V1 is a part of an ion pump V-ATPase, which transports cations across the membrane by ATP-hydrolysis-driven rotation. V1 comprises a rotor composed of the D and F subunits, and a stator, a hexameric ring, composed of three A subunits and three B subunits. However, the details of their sequences and structures are different, resulting in two different interfaces between the A and B subunits in the A3B3 hexameric ring: a catalytic interface, at which the A subunit has an ATP-hydrolysis catalytic site; and a non-catalytic interface, at which the B subunit has a pseudo-active site, which has evolutionally lost the ATP-hydrolysis or even binding ability. We used computational design to restore the lost ATP-binding ability of the pseudo-active site in the B subunit of a rotary molecular motor, V1-ATPase.

The designed B subunit (De), expressed together with the A subunit in Escherichia coli and purified by Ni2+-affinity chromatography followed by gel-filtration chromatography, was found to form a ring complex with the A subunit (A3(De)3 ring complex). Therefore, we determined the crystal structures of the A3(De)3 complex to prove the nucleotide-binding ability of De. First, the A3(De)3 complex was crystallized in the absence of nucleotide and the structure was solved at 2.8 Å resolution; this was named A3(De)3_empty. The De structure in A3(De)3_empty was almost identical to the computational model not only in terms of the overall structure but also in terms of the designed site together with the P-loop features. ADP molecules are shown as spheres. c,d, Superposition of the computational design model of the designed B subunit (white) and the solved crystal structure in the absence of nucleotides (pink) (chain D of A3(De)3_empty was used because this had the highest resolution data of the three designed B subunits): comparison for the entire backbone (the Cα r.m.s.d. calculated by MICAN33 is 1.48 Å) (c); comparison for the designed binding site (d). The backbone geometry of the designed P-loop was almost identical to that of the design model. e, The interface between chains C and D in A3(De)3_(ADP·Pi)1cat(ADP)2cat,2non-cat.

>SSGMQIGKIIKVSGPLVMAENMSEASIQDMCLVGDLGVIGEIIEMRQDVASIQVYEETSGIGPGEPVRSTGEALSVELGPGIISQMFDGIQRPLDTFMEVTQSNFLGRGVQLPALDHEKQWWFEATIEEGTEVSAGDIIGYVDETKIIQHKIMVPNGIKGTVQKIESGSFTIDDPICVIETEQGLKELTMMQKWPVRRGRPIKQKLNPDVPMITGQRVIDTFFPVTKGGAAAVPGPFGAGKTVVQHQIAKWSDVDLVVYVGCGERGNEMTDVVNEFPELIDPNTGESLMERTVLIANTSNMPVAAREASIYTGITIAEYFRDMGYDVAIMADSTSRWAEALREMSGRLEEMPGDEGYPAYLGSRLAEYYERSGRVIALGSDQREGSITAISAVSPSGGDISEPVTQNTLRVVKVFWGLDSSLAQKRHFPSINWIQSYSLYSTEVGRYMDQILQQDWSDMVTEGMRILQEEEQLNEIVRLVGIDSLSDNDRLTLEVAKSIREDYLQQNAFDDVDTFTSREKQFNMLKVILTFGKEARKALSLGAYFNEIMEGTVAVRERISRSKYIPEEELAKISSINEEIKETIQLIVSEGGMTDD[3x];>[3x]MIKEYRTIKEVVGPLMAVEKVSGVKYEELIEVRMQNGEIRRGQVLEVQEDKAMVQIFEGTSGINLKNSSVRFLGHPLQLGVSEDMIGRVFDGLGRPKDNGPEILPEKYLDINGEVINPIARDYPDEFIQTGISAIDHLNTLVRGQKLPVFGPPGAGKSALAAQIARQATVLDSSDDFAVVFAAIGITFEEAEFFMEDFRQTGAIDRSVMFMNLANDPAIERIATPRMALTAAEYLAYEKGMHVLVIMEDMTNYAEALREISAARREVPGRRGYPGYLYTNLATLFERAGRIRGLKGSVTQIPILTMPEDDKTHPIPDLTGYITEGQIILTRELYKSGISPPIDVLPSLSRLKDKGTGAGKTREDHAATMNQLFAAYAQGKQAKELAVVLGESALSDIDKIYAKFAERFENEYVNQGFYTNRTITETLDLGWELLAMLPRTELKRIKDDLLDKYLPEGK>[6x]MSLSQPIYKRILLKLSGEALQGEDGLGIDPAILDRMAVEIKELVEMGVEVSVVLGGGNLFRGAKLAKAGMNRVVGDHMGMLATVMNGLAMRDSLFRADVNAKLMSAFQLNGICD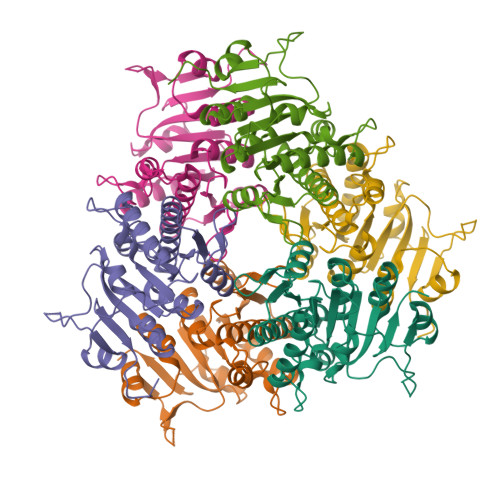TYNWSEAIKMLREKRVVIFSAGTGNPFFTTDSTACLRGIEIEADVVLKATKVDGVYDCDPAKNPDAKLYKNLSYAEVIDKELKVMDLSAFTLARDHGMPIRVFNMGKPGALRQVVTGTEEGTTICEGHHHHHH> RLFPPQWICCDIRYLDVSILGKFAVVMADPPWDIHMELPYGTLTDDEMRRLNIPVLQDDGFLFLWVTGRAMELGRECLNLWGYERVDEIIWVKTNQLQRIIRTGRTGHWLNHGKEHCLVGVKGNPQGFNQGLDCDVIVAEVRSTSHKPDEIYGMIERLSPGTRKIELFGRPHNVQPNWITLGNQLDGIHLLDPDVVARFKQRYPDGIISKP;> NDYCQHFVDTGHRPQNFIRDVGLADRFEEYPKLRELIRLKDELIAKSNTPPMYLQADIEAFDIRELTPK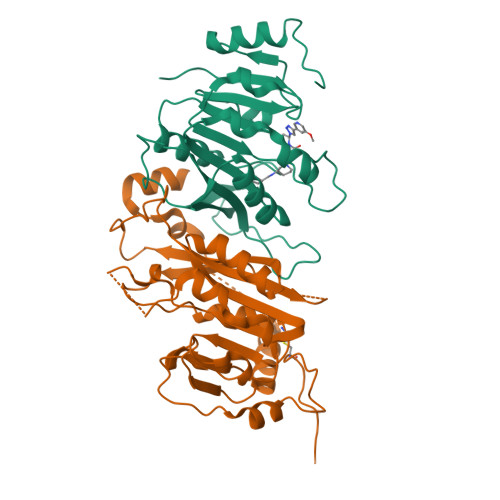FDVILLEPPLEEYYRETGITANEKCWTWDDIMKLEIDEIAAPRSFIFLWCGSGEGLDLGRVCLRKWGYRRCEDICWIKTNKNNPGKTKTLDPKAVFQRTKEHCLMGIKGTVKRSTDGDFIHANVDIDLIITEEPEIGNIEKPVEIFHIIEHFCLGRRRLHLFGRDSTIRPGWLTVGPTLTNSNYNAETYASYFSAPNSYLTGCTEEIERL(10ALPHA,13ALPHA,14BETA,17ALPHA)-17-HYDROXYANDROST-4-EN-3-ONE 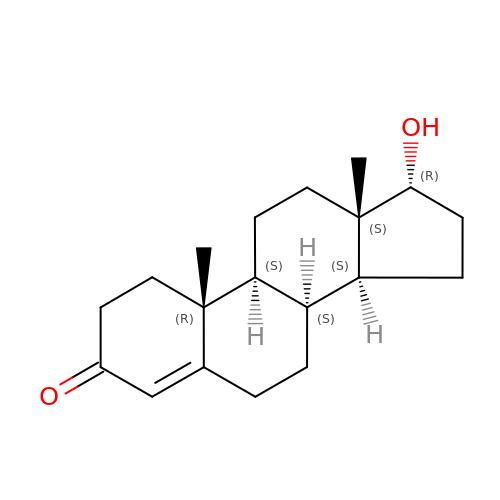| C19 H28 O2 | MUMGGOZAMZWBJJ-KZYORJDKSA-N> SDRIIQITRGDSTITSQDVANAVVGYGVWPHYLTPQDATAIDKPTQPDTSSNRFYTLDSKMWNSTSKGWWWKLPDALKDMGIFGENMFYHFLGRSGYTVHVQCNASKFHQGTLLVVMIPEHQLATVNKGNVNAGYKYTHPGEAGREVGTQVENEKQPSDDNWLNFDGTLLGNLLIFPHQ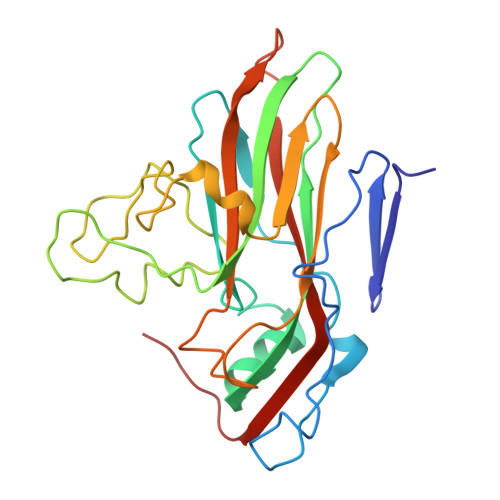FINLRSNNSATLIVPYVNAVPMDSMVRHNNWSLVIIPVCQLQSNNISNIVPITVSISPMCAEFSGARAKTVVQ>MSHLAELVASAKAAISQASDVAALDNVRVEYLGKKGHLTLQMTTLRELPPEERPAAGAVINEAKEQVQQALNARKAELESAALNARLAAETIDVSLPGRRIENGGLHPVTRTIDRIESFFGELGFTVATGPEIEDDYHNFDALNIPGHHPARADHDTFWFDTTRLLRTQTSGVQIRTMKAQQPPIRIIAPGRVYRNDYDQTHTPMFHQMEGLIVDTNISFTNLKGTLHDFLRNFFEEDLQIRFRPSYFPFTEPSAEVDVMGKNGKWLEVLGCGMVHPNVLRNVGIDPEVYSGFAFGMGMERLTMLRYGVTDLRSFFENDLRFLKQFK[2x];>MKFSELWLREWVNPAIDSDALANQITMAGLEVDGVEPVAGSFHGVVVGEVVECAQHPNADKLRVTKVNVGGDRLLDIVCGAPNCRQGLRVAVATIGAVLPGDFKIKAAKLRGEPSEGMLCSFSELGISDDHSGIIELPADAPIGTDIREYLKLDDNTIEISVTPNRADCLGIIGVARDVAVLNQLPLVQPEIVPVGATIDDTLPITVEAPEACPRYLGRVVKGINVKAPTPLWMKEKLRRCGIRSIDAVVDVTNYVLLELGQPMHAFDKDRIEGGIVVRMAKEGETLVLLDGTEAKLNADTLVIADHNKALAMGGIFGGEHSGVNDETQNVLLECAFFSPLSITGRARRHGLHTDASHRYERGVDPALQHKAMERATRLLIDICGGEAGPVIDITNEATLPKRATITLRRSKLDRLIGHHIADEQVTDILRRLGCEVTEGKDEWQAVAPSWRFDMEIEEDLVEEVARVYGYNNIPDEPVQASLIMGTHREADLSLKRVKTLLNDKGYQEVITYSFVDPKVQQMIHPGVEALLLPSPISVEMSAMRLSLWTGLLATVVYNQNRQQNRVRIFESGLRFVPDTQAPLGIRQDLMLAGVICGNRYEEHWNLAKETVDFYDLKGDLESVLDLTGKLNEVEFRAEANPALHPGQSAAIYLKGERIGFVGVVHPELERKLDLNGRTLVFELEWNKLADRVVPQAREISRFPANRRDIAVVVAENVPAADILSECKKVGVNQVVGVNLFDVYRGKGVAEGYKSLAISLILQDTSRTLEEEEIAATVA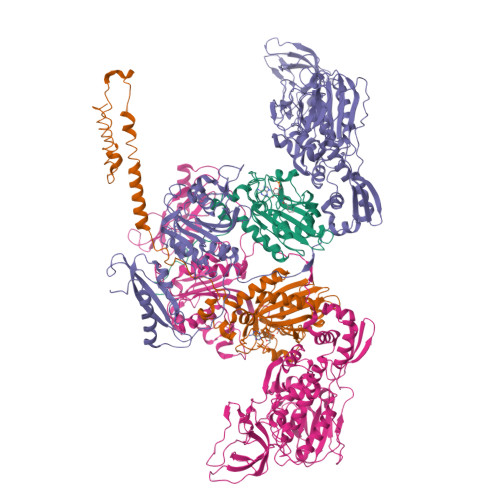KCVEALKERFQASLRD[2x]1-(N-BENZYLOXYCARBONYL-L-LEUCINYL)-5-(3-BENZYLOXY 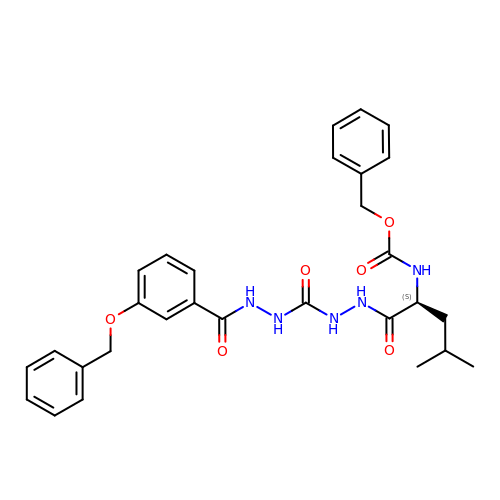BENZOYL)CARBOHYDRAZIDE | C29 H33 N5 O6 | CEXWCIXCWCFUSI-VWLOTQADSA-N>MKKLLPILIGLSLSGFSSLSQAENLMQVYQQARLSNPELRKSAADRDAAFEKINEARSPLLPQLGLGADYTYSNGYRDANGINSNATSASLQLTQSIFDMSKWRALTLQEKAAGIQDVTYQTDQQTLILNTATAYFNVLNAIDVLSYTQAQKEAIYRQLDQTTQRFNVGLVAITDVQNARAQYDTVLANEVTARNNLDNAVEQLRQITGNYYPELAALNVENFKTDKPQPVNALLKEAEKRNLSLLQARLSQDLAREQIRQAQDGHLPTLDLTASTGISDTSYSGSKTRGAAGTQYDDSNMGQNKVGLSFSLPIYQGGMVNSQVKQAQYNFVGASEQLESAHRSVVQTVRSSFNNINASISSINAYKQAVVSAQSSLDAMEAGYSVGTRTIVDVLDATTTLYNAKQELANARYNYLINQLNIKSALGTLNEQDLLALNNALSKPVSTNPENVAPQTPEQNAIADGYAPDSPAPVVQQTSARTTTSNGHNPFRN[3x];>MRYSKLTMLIPCALLLSACTTVTPAYKDNGTRSGPCVEGGPDN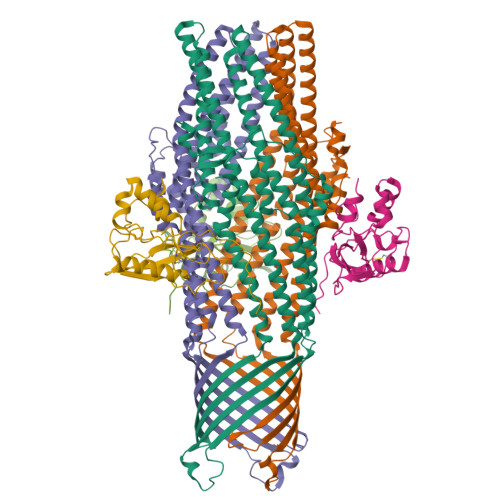VAQQFYDYRILHRSNDITALRPYLSDKLATLLSDASRDNNHRELLTNDPFSSRTTLPDSAHVASASTIPNRDARNIPLRVDLKQGDQGWQDEVLMIQEGQCWVIDDVRYLGGSVHATAGTLRQSIENR[3x]> GMMYTNDNRIVMTLDAGGTNFVFSAIQGGKEIADPVVLPACADCLDKCLGNLVEGFKAIQAGLPEAPVAISFAFPGPADYQAGIIGDLPNFPSFRGGVALGPFLEDIFGIPVFINNDGSLFAYGEALTGVLPEINRRLREAGSTKRYKNLLGVTLGTGFGAGVVIDGE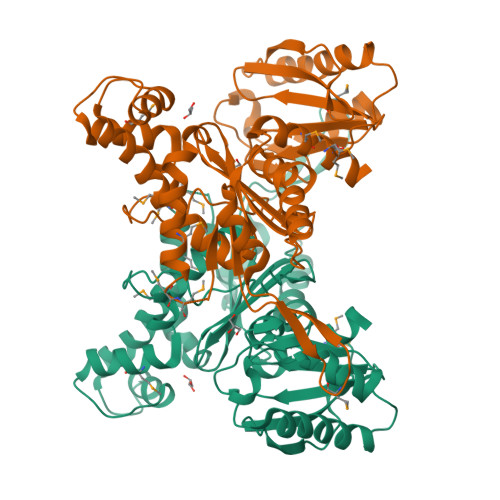LLRGDNAAGGYVWCLRNKKYPEYIVEESVSIRAVMRVYAERSGDAGARTPKEIFEIAEGIRPGNREAAIAAFEELGEMAGDALASAITLIDGLIVIGGGLSGASKYILPVLLKEMNAQTGMMDGARFGRLQKEVYDLDEEKSFAGFARGEAVEVLVPGTNRKVGYDPCKRIGVTFSKQGANRSIAMGAYVFALNHLSK>[2x]MGGSSHHHHHHSSGLVPRGSHMKLITASSSKEYLPDLLLFWQNYEYWITNIGLYKTKQRDLTRTPANLDTDTEECMFWMNYLQKDQSFQLMNFAMENLGALYFGSIGDISELYLRVEQYWDRRADKNHSVDGKYWDALIWSVFTMCIYYMPVEKLAEIFSVYPLHEYLGSNKRLNWEDGMQLVMCQNFARCSLFQ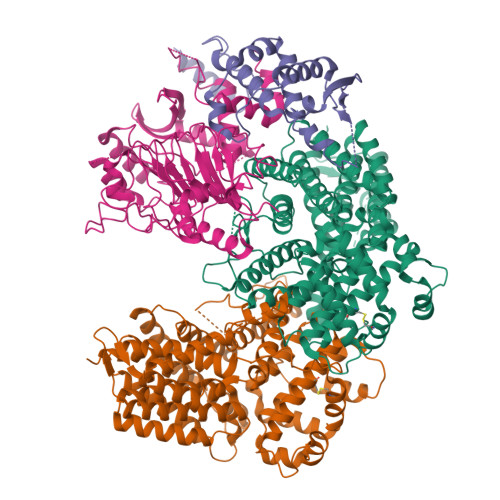LKQCDFMAHPDIRLVQAYLILATTTFPYDEPLLANSLLTQCIHTFKNFHVDDFRPLLNDDPVESIAKVTLGRIFYRLCGCDYLQSGPRKPIALHTEVSSLLQHAAYLQDLPNVDVYREENSTEVLYWKIISLDRDLDQYLNKSSKPPLKTLDAIRRELDIFQYKVDSLEEDFRSNNSRFQKFIALFQISTVSWKLFKMYLIYYDTADSLLKVIHYSKVIISLIVNNFHAKSEFFNRHPMVMQTITRVVSFISFYQIFVESAAVKQLLVDLTELTANLPTIFGSKLDKLVYLTERLSKLKLLWDKVQLLDSGDSFYHPVFKILQNDIKIIELKNDEMFSLIKGLGSLVPLNKLRQESLLEEEDENNTEPSDFRTIVEEFQSEYNISDILS;> MGVTSNVVLVSGEGERFTVDKKIAERSLLLKNYLNDMHDSNLQNNSDSESDSDSETNHKSKDNNNGDDDDEDDDEIVMPVPNVRSSVLQKVIEWAEHHRDSNFPDEDDDDSRKSAPVDSWDREFLKVDQEMLYEIILAANYLNIKPLLDAGCKVVAEMIRGRSPEEIRRTFNIVNDFTPEEEAAIRRENEWAEDRGS;> MGPSFNPVRFLELPIDIRKEVYFHLDGNFCGAHPYPIDILYKSNDVELPGKPSYKRSKRSKKLLRYMYPVFATYLNIFEYSPQLIEKWLEYAFWLRYDCLVLDCFKVNHLYDGTLIDALEWTYLDNELRLAYFNKASMLEVWYTFKEYKKWVIDSVAFDELDLLNVSNIQFNIDNLTPQLVDKCLSILEQKDLFATIGEVQFGQDEEVGEEKDVDVSGANSDENSSPSSTIKNKKRSASKRSHSDNGNVGATHNQLTSISVIRTIRSMESMKSLRKITVRGEKLYELLINFHGFRDNPGKTISYIVKRRINEIRLSRMNQISRTGLADFTRWDNLQKLVLSRVAYIDLNSIVFPKNFKSLTMKRVSKIKWWNIEENILKELKVDKRTFKSLYIKEDDSKFTKFFNLRHTRIKELDKSEINQITYLRCQAIVWLSFRTLNHIKLQNVSEVFNNIIVPRALFDSKRVEIYRCEKISQVLVIGSRSGSENLYFQGSKRRWKKNFIAVSAANRFKKISSSGAL5-(2-Morpholin-4-yl-7-pyridin-3-yl-6,7-dihydro-5H-pyrrolo[2,3-d]pyrimidin-4-yl)-pyrimidin-2-ylamine 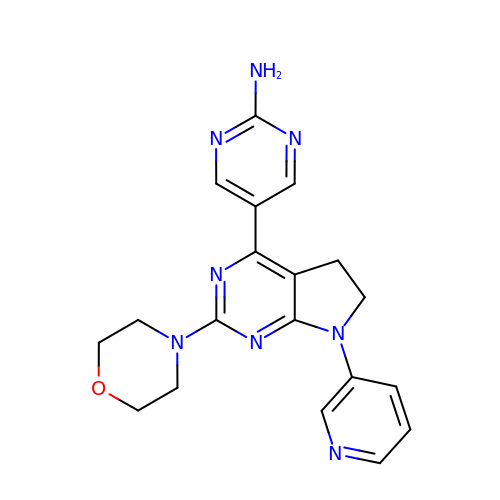| C19 H20 N8 O | WZVLQVVHYKFKAZ-UHFFFAOYSA-N> FVG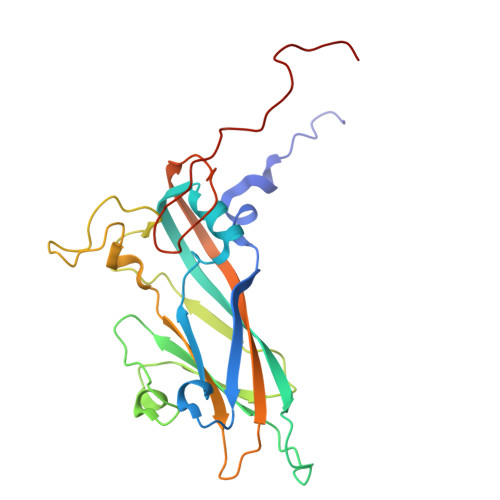GFHTRSESSLENFLGRAANTYRTSFKTLSTKPSLKFASWTITTRKVAMLRRKMEMFTYMRFDVEVTFVITSSKCKSDPSSGSLPVLTFMVQYVPPGGPVPSSVDSFSWQSSTNPSIFWTQGNAPPRMSIPYMSIGNAYSNYYDGYSHHGADGVYGYNTLNNQGQLYFRHVNSSNPGAYTCVVKIYFKLQHVKAWVPRPPRLCNYQRAENVNFKVQGVTDTKESITANPG>[2x]ATCDDGRTTANAACCILFPILDDIQENLFDG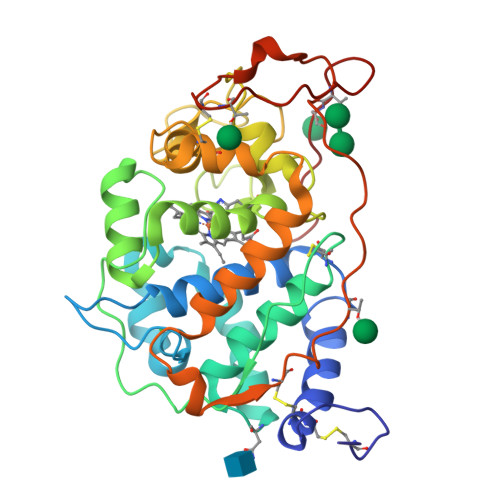AQCGEEVHESLRLTFHDAIGFSPTLGGGGADGSIIAFDTIETNFPANAGIDEIVSAQKPFVAKHNISAGDFIQFAGAVGVSNCPGGVRIPFFLGRPDAVAASPDHLVPEPFDSVDSILARMGDAGFSPVEVVWLLASHSIAAADKVDPSIPGTPFDSTPGVFDSQFFIETQLKGRLFPGTADNKGEAQSPLQGEIRLQSDHLLARDPQTACEWQSMVNNQPKIQNRFAATMSKMALLGQDKTKLIDCSDVIPTPPALVGAAHLPAGFSLSDVEQACAATPFPALTADPGPVTSVPPVPGS>[2x]GSVVIGQRCYRSPD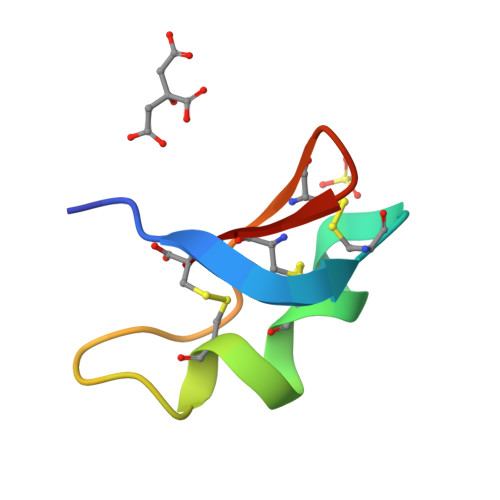CYSACKKLVGKATGKCTNGRCDC> IPALKANGQLEVDGKRYEIRAADDGTISVLRPEQQSKAKSFFKGA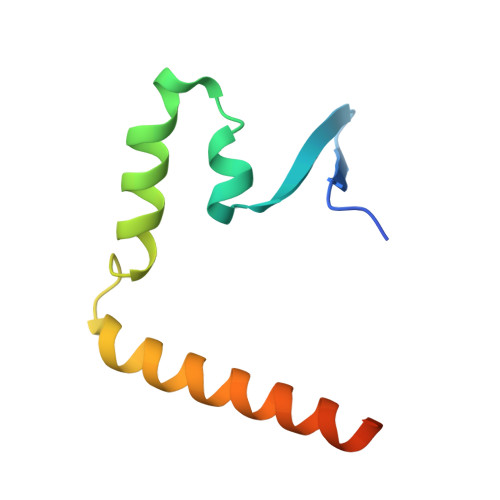SQLIGGSSQRAQIAQALNEKVASARTVLHQSAMTGGR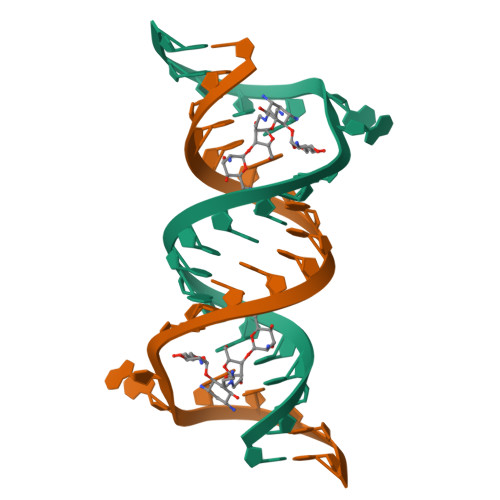>[2x]CGCGUCACACCGGUGAAGUCGC>MSGADRSPNAGAAPDSAPGQAAVASAYQRFEPRAYLRNNYAPPRGDLCNPNGVGPWKLRCLAQTFATGEVSGRTLIDIGSGPT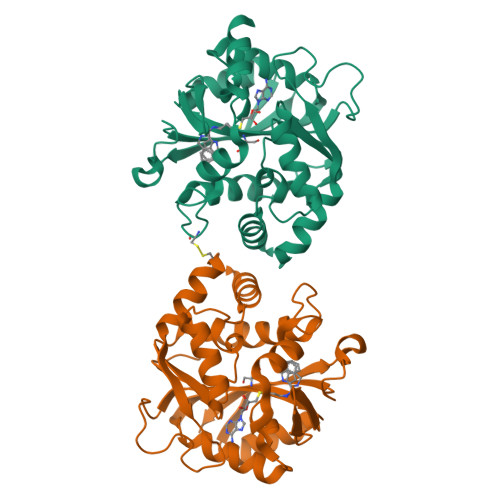VYQLLSACSHFEDITMTDFLEVNRQELGRWLQEEPGAFNWSMYSQHACLIEGKGECWQDKERQLRARVKRVLPIDVHQPQPLGAGSPAPLPADALVSAFCLEAVSPDLASFQRALDHITTLLRPGGHLLLIGALEESWYLAGEARLTVVPVSEEEVREALVRSGYKVRDLRTYIMPAHLQTGVDDVKGVFFAWAQKVGLEHHHHHH[2x]> YKQLQLQERTNIRKCQELLEQLNGKINLTYRADF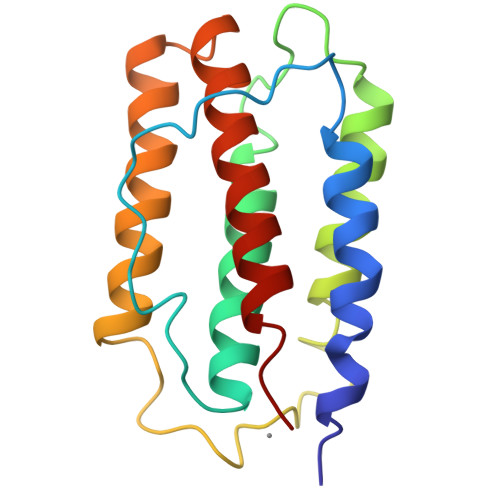KIPMEMTEKMQKSYTAFAIQEMLQNVFLVFRNNFSSTGWNETIVVRLLDELHQQTVFLKTVLEEKQEERLTWEMSSTALHLKSYYWRVQRYLKLMKYNSYAWMVVRAEIFRNFLIIRRLTRNFQ>[2x]GASHPEIEKAQREIIEAFNAKPKNGINKIKEICEQYKISPNEEIAEFFHQQRKNLDLEAVGDYLSSPEAENQQVLKAFTSQMNFNGQSFVEGLRTFLKTFKLPGEAQKIDRLVQSFSGAYFQQNPDVVSNADAAYLLAFQTIMLNTDLHNPSI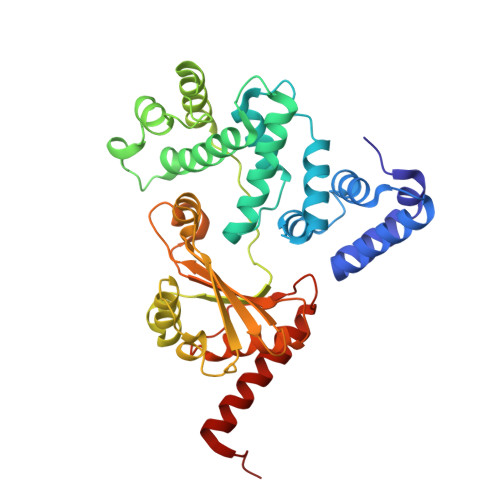PEKNKMTVDGLKRNLRGGNNGGDFDAKFLEELYSEIKAKPFELNFVKTSPGYELTSTTLNKDSTFKKLDSFLHSTDVNINTVFPGIGDNVKTTVDQPKSWLSFFTGYKGTITLTDNKTSAQATIQVYTPNIFSKWLFGEQPRVIIQPGQTKESIDLAAKAAADFSSPVKNFKATYDYEVGDLIKAYDNQKKLITIERNLALKA> GAMGTEKVLQICPKDMRADICVHLNRKVFKEHPAFRLASDGCLRALAMEFQTVHCAPGDLIYHAGESVDSLCFVVSGSLEVIQDD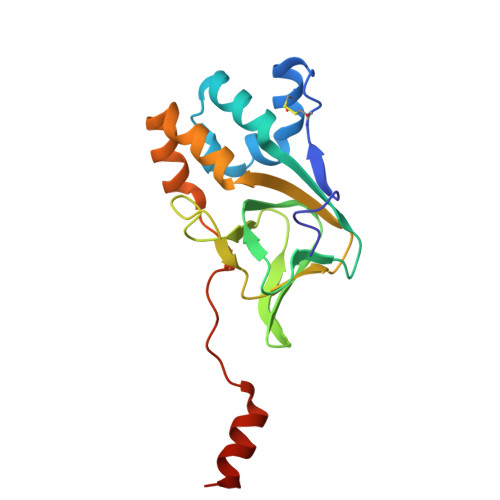EVVAILGKGDVFGDVFWKEATLAQSCANVRALTYCDLHVIKRDALQKVLEFYTAFSHSFSRNLILTYNLRKRIVFRKISDVKREEEERMKRK Soluble HMW1C-like N-glycosyltransferases (NGTs) catalyze the glycosylation of Asn residues in proteins, a process fundamental for bacterial autoaggregation, adhesion and pathogenicity. In contrast, NGTs are two-domain enzymes that consists of an N-terminal all-α domain (AAD) and a C-terminal catalytic domain that adopts a GT-B fold, as shown for Actinobacillus pleuropneumoniae NGT (ApNGT). We focused on AaNGT, an inverting GT that catalyzes the transfer of Glc from UDP-Glc to Asn residues in the consensus sequence Asn-X-Ser/Thr. The heart-shaped structure of AaNGT, either complexed to UDP-Gal/UDP-2F-Glc or UDP-peptide, shows the N-terminal AAD domain and C-terminal GT-B fold catalytic domain, which is composed of an N- and C-Rossman fold subdomains.

Having characterized AaNGT with different sugar nucleotides, UDP, and the peptide FGNWTT, we obtained P212121 crystals of AaNGT in complex with UDP-Gal, UDP-2F-Glc, and UDP plus the peptide. Overall, our results of kinetic and binding experiments indicate that UDP-Glc is a preferred substrate of AaNGT compared to UDP-Gal, whereas UDP-Glc mimetics act as inhibitors of the enzyme. In contrast, the UDP-Gal and UDP-2F-Glc pyrophosphates are only recognized by the side chains of Lys440 and Asn520. The sugar molecules interact with the side chains of His276 and Ser277. Furthermore, the Gal moiety specifically interacts with the Gly369 backbone, while the 2F-Glc moiety interacts with the side chain of His370. The superposition of all ligands for all three structures (AaNGT/UDP, AaNGT/UDP-Gal, and AaNGT/UDP-2F-Glc) clearly shows that the sugar moieties of UDP-Gal and UDP-2F-Glc collide with Gly2-1 and Asn30. This suggests that the sugar nucleotides adopt unproductive conformations in their respective enzyme complexes, which could explain why we were unable to get a ternary complex resembling a Michaelis complex at a structural level. Furthermore, this could also explain why UDP-Gal is a poor substrate, and UDP-Glc mimetics are inhibitors of AaNGT. The interaction of the 2-OH and the β-phosphate group could explain why the enzyme cannot recognize UDP−2F-Glc in a productive manner. Likewise, the interactions between OH3 and OH4 of Glc with Leu368 could explain the poor interaction with UDP-Gal. The results of our ITC experiments demonstrated that the product of the reaction, UDP, binds to AaNGT ~ 3–5.8-fold and 18-fold better than UDP-Glc mimetics and UDP-Gal, respectively.

>GMSRKKNPSVIQFEKAITEKNYEAACTELLDILNKIDTNFGDIEGIDFDYPQQLETLMQDRIVYFCTRMSNAITQLFCDPQFSLSESGANRFFVVQRWLNLIFASSPYINADHILQTYNCNPERDSIYDIYLEPNKNVLMKFAVLYLPESNVNLNLDTMWETDKNICGSLCFALQSPRFIGTPAAFSKRSTILQWFPAKLEQFHVLDDLPSNISHDVYMHCSYDTAENKHNVKKALNQVIRSHLLKCGWQDRQITQIGMRNGKPVMVVVLEHFHSSHSIYRTHSTSMIAAREQFYLIGLGNNAVDQAGRDVFDEFHEFDGSNILKKLAFLKEMCEKNDAAVLYMPSIGMDLATIFVSNARFAPIQVIALGHPATTHSEFIEYVIVEDDYVGSESCFSETLLRLPKDALPYVPSSLAPTDVQYVLRETPEVVNIGIAATTMKLNPYFLETLKTIRDRAKVKVHFHFALGQSIGITHPYVARFIRSYLGDDATAHPHSPYNRYLDILHNCDMMLNPFPFGNTNGIIDMVTLGLVGVCKTGPEVHEHIDEGLFKRLGLPEWLIADSVEDYIERAIRLAENHQERLALRRHIIENNGLKTLFSGDPSPMGKTLFAKLTEWRQTNGI[2x]~{N}-[5-[[4-[bis(fluoranyl)methoxy]phenyl]sulfamoyl]-2-chloranyl-phenyl]-3,5-bis(fluoranyl)benzamide 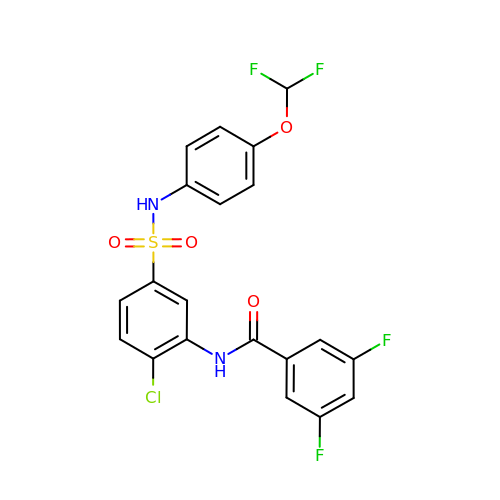| C20 H13 Cl F4 N2 O4 S | NAGQOJQGBKEXGZ-UHFFFAOYSA-N>MGHHHHHHSHMGSEIGTGFPFDPHYVEVLGERMHYVDVGPRDGTPVLFLHGNPTSSYLWRNIIPHVAPSHRCIAPDLIGMGKSDKPDLDYFFDDHVRYLDAFIEALGLEEVVLVIHDWGSALGFHWAKRNPERVKGIACMEFIRPIPTWDEWPEFARETFQAFRTADVGRELIIDQNAFIEGALPMGVVRPLTEVEMDHYREPFLKPVDREPLWRFPNELPIAGEPANIVALVEAYMNWLHQSPVPKLLFWGTPGVLIPPAEAARLAESLPNCKTVDIGPGLFLLQEDNPDLIGSEIARWLPG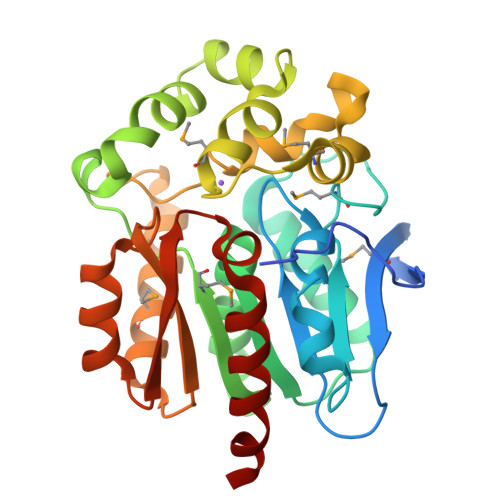LAG[2x]> MTVF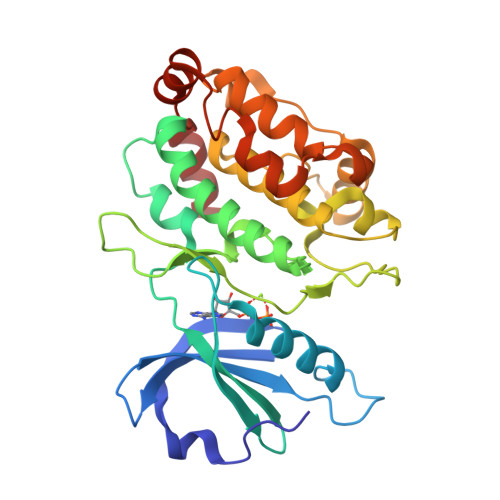RQENVDDYYDTGEELGSGQFAVVKKCREKSTGLQYAAKFIKKRRTKSSRRGVSREDIEREVSILKEIQHPNVITLHEVYENKTDVILILELVAGGELFDFLAEKESLTEEEATEFLKQILNGVYYLHSLQIAHFDLKPENIMLLDRNVPKPRIKIIDFGLAHKIDFGNEFKNIFGTPEFVAPEIVNYEPLGLEADMWSIGVITYILLSGASPFLGDTKQETLANVSAVNYEFEDEYFSNTSALAKDFIRRLLVKDPKKRMTIQDSLQHPWIKPKDTQQALSRKASAVNMEKFKKFAAR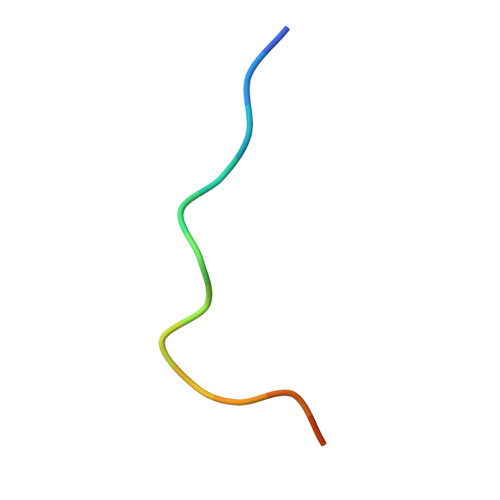> DLSPRPSPNPHPVSQ>[2x]MPLTKQDAVNQMMGFFQAKALTAALALKLFDQLRDRDADAAHIAARLDCPARSTEQLLIALRAMGYLDQRDGLYHLPAAHRAFLLSDEPQWLGWLGRHIDTFLYPLWGELKTAVRNDAHQRRTVFGDDRSWFDILYQNPDDVADFQEFLGKFAAPFIAGFVRDYDFSQHRAFLDIGSGIGSLPMAIADAYPGIALAICELPQASAFLRDKLTLQGYGERIDVVEGDVISGDLPIGGYDLIHLG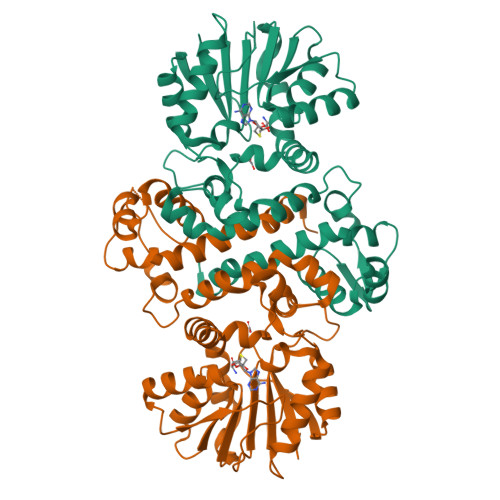WMLHDYAPETQLTILRNIYRAMPAGGRFIASETPLNEDKSGPEFTALLSLNMLVSTDGGIESSAQEYLDRFRLAGFSNARIMKIAGPRTLIVGEKLEHHHHHH>[4x]EEEGRIRAMRAARSLGERTVTELILQHQNPQQLSSNLWAAVRARGCQFLGPAMQEEALKLVLLALEDGSALSRKVLVLFVVQRLEPRFP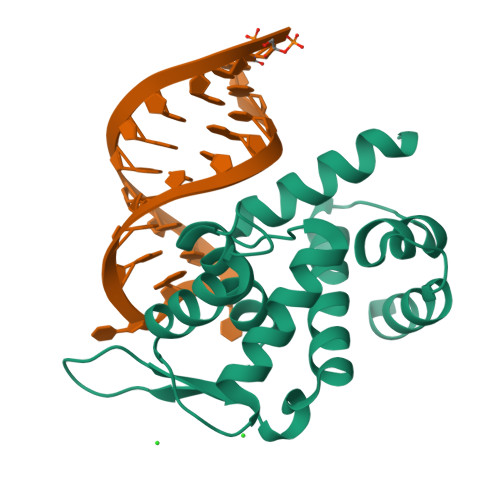QASKTSIGHVVQLLYRASCFKVTKRDEDSSLMQLKEEFRTYEALRREHDSQIVQIAMEAGLRIAPDQWSSLLYGDQSHKSHMQSIIDKLQT>[4x]MGRIKNKQFAVIGLG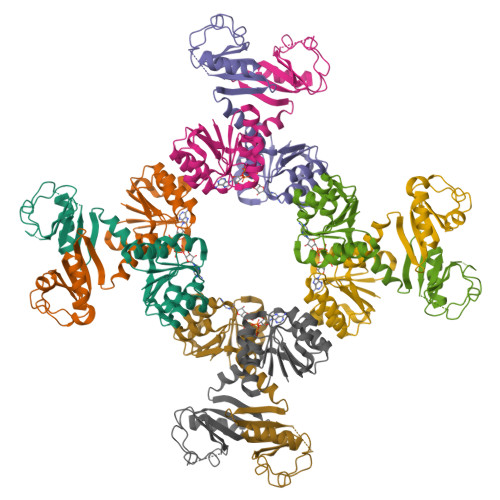RFGGSICKELHRMGHEVLAVDINEEKVNAYASYATHAVIANATEENELLSLGIRNFEYVIVAIGANIQASTLTTLLLKELDIPNIWVKAQNYYHHKVLEKIGADRIIHPEKDMGVKIAQSLSDENVLNYIDLSDEYSIVELLATRKLDSKSIIDLNVRAKYGCTILAIKHHGDICLSPAPEDIIREQDCLVIMGHKKDIKRFENEGM> MKNPLVVLLGFV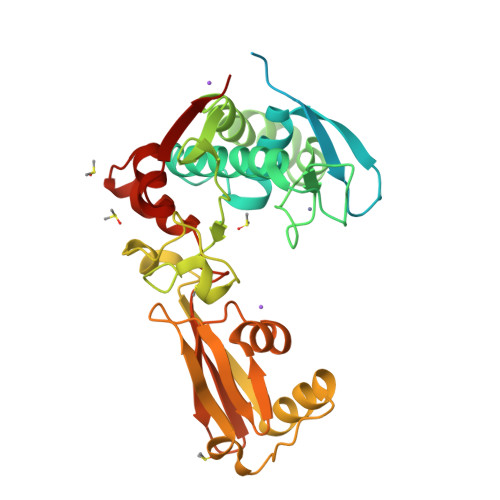TCSVLVPSLITLVSYKNVELTEKPESPVSINKTIKKSDIEDKGNKEEKNTVNYETVNKKAPIINVYNHITGKTEKMDMENYLCGVLAGEMSSEFDIEALKAQSVAARTYVVYKQEHGKSSKHKNAVVCTDYKHCQEYKSYDTLKKLNGEEWIKNKYSKIQEAVRGTKGQIITYNDKAILPLYFSTSSGKTENSEEVFSAKYPYLKSVESPYDKYSPKFASTLKISNTDFVKSLRRAYSTIVIDVNNLSKQVSITKRSDAGTVEKIKLGNKELTGKDIRTVFKLNSANFDIKFGEGYIDFVVKGYGHGVGMSQWGAEGMAEEGYKYYDILSHYYTDTKIKDIY>[4x]MTPDELNSAVVTFMANLNIDDSKANETASTVTDSIVHRSIKLLEVVVALKDYFLSENEVERKKALTCLTTILAKTPKDHLSKNECSVIFQFYQSKLDDQALAKEVLEGFAALAPMKYVSINEIAQLLRLLLDNYQQGQHLASTRLWPFKILRKIFDRFFVNGSSTEQVKRINDLFIETFLHVANGEKDPRNLLLSFALNKSITSSLQNVENFKEDLFDVLFCYFPITFKPPKHDPYKISNQDLKTALRSAITATPLFAEDAYSNLLDKLTASSPVVKNDTLLTLLECVRKFGGSSILENWTLLWNALKFEIMQNSEGNENTLLNPYNKDQQSDDVGQYTNYDACLKIINLMALQLYNFDKVSFEKFFTHVLDELKPNFKYEKDLKQTCQILSAIGSGNVEIFNKVISSTFPLFLINTSEVAKLKLLIMNFSFFVDSYIDLFGRTSKESLGTPVPNNKMAEYKDEIIMILSMALTRSSKAEVTIRTLSVIQFTKMIKMKGFLTPEEVSLIIQYFTEEILTDNNKNIYYACLEGLKTISEIYEDLVFEISLKKLLDLLPDCFEEKIRVNDEENIHIETILKIILDFTTSRHILVKESITFLATKLNRVAKISKSREYCFLLISTIYSLFNNNNQNENVLNEEDALALKNAIEPKLFEIITQESAIVSDNYNLTLLSNVLFFTNLKIPQAAHQEELDRYNELFISEGKIRILDTPNVLAISYAKILSALNKNCQFPQKFTVLFGTVQLLKKHAPRMTETEKLGYLELLLVLSNKFVSEKDVIGLFDWKDLSVINLEVMVWLTKGLIMQNSLESSEIAKKFIDLLSNEEIGSLVSKLFEVFVMDISSLKKFKGISWNNNVKILYKQKFFGDIFQTLVSNYKNTVD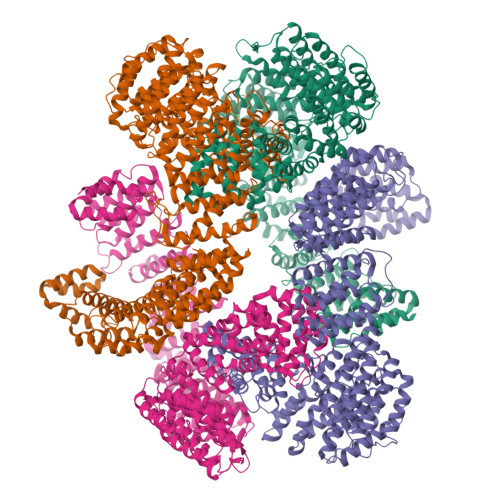MTIKCNYLTALSLVLKHTPSQSVGPFINDLFPLLLQALDMPDPEVRVSALETLKDTTDKHHTLITEHVSTIVPLLLSLSLPHKYNSVSVRLIALQLLEMITTVVPLNYCLSYQDDVLSALIPVLSDKKRIIRKQCVDTRQVYYELGQIPFE Leucine-rich repeat-containing G protein-coupled receptor 4 (LGR4) plays a critical role in regulating the wingless-related integration site (Wnt) signaling pathway and is essential for organ development and carcinogenesis. LGR4, along with its ligand R-spondin (RSPO), potentiates Wnt/β-catenin signaling by recruiting its signaling suppressor, E3 ligase Zinc and Ring Finger 3 (ZNRF3), and inducing its membrane clearance. Cell surface-expressed LGR4/5, members of the class A G-protein coupled receptors (GPCR) family, have an extracellular domain (ECD) comprising 17 leucine-rich repeats (LRRs), followed by a seven-transmembrane domain (TMD), and an intracellular domain (ICD). ZNRF3/RNF43, LGR4, and RSPO form a ternary complex on the cell surface, which relieves ZNRF3/RNF43-mediated suppression of Wnt/β-catenin signaling and thereby potentiates pathway activation.

We purified LMNG/CHS detergent-solubilized ternary complexes of human LGR4, RSPO2, and ZNRF3 (residues 56-267, ECD-TMD) from Expi293F cells cotransfected with LGR4, RSPO2, and ZNRF3. Cryo-EM analysis of this sample revealed two distinct LGR4–RSPO2–ZNRF3 complexes with stoichiometric ratios of 1:1:2 and 2:2:2, corresponding to a heterotetramer and a heterohexamer, respectively. We obtained cryo-EM maps of LGR4-RSPO2-ZNRF31:1:2 heterotetramer and LGR4-RSPO2-ZNRF32:2:2 heterohexamer to resolutions of 3.2 Å and 3.5 Å, respectively. In the LGR4-RSPO2-ZNRF32:2:2 complex, another copy of the LGR4*-RSPO2* complex was bound to the other protomers of the ZNRF3 dimer, ZNRF3* (the asterisk indicates the second protomer in the dimer), forming another set of 1:1:1 complexes, thus completing the C2-symmetrical 2:2:2 complex. In the LGR4-RSPO2-ZNRF32:2:2 complex, the TM helices of ZNRF3 protomers were visible in the cryo-EM density. The two TM helices of ZNRF3 were loosely sandwiched between the two TMDs of LGR4, especially between TM1 and TM7 of one LGR4 promoter and TM6 of the other LGR4* promoter. The two TM helices of ZNRF3 made contact with each other at a distance of 5–7 Å on the extracellular side of the membrane. In addition to the ECD dimerization of ZNRF3, these intermolecular contacts in the membrane restrict the spatial positioning of the TM helices of ZNRF3 and bring the intracellular region of ZNRF3 into proximity, which may facilitate the auto-ubiquitination of ZNRF320,28,29. In the 2:2:2 heterohexamer configuration, ZNRF3 ECD and TMD are largely enclosed by LGR4 and RSPO2, resulting in steric hindrance that prevents ZNRF3 from binding to the FZDs, thereby suppressing its ubiquitination activity. Moreover, no apparent contact was observed between the two LGR4 protomers within the 2:2:2 heterohexamer.

>[2x]MPGPLGLLCFLALGLLGSAGPSGAAPPLCAAPCSCDGDRRVDCSGKGLTAVPEGLSAFTQALDISMNNITQLPEDAFKNFPFLEELQLAGNDLSFIHPKALSGLKELKVLTLQNNQLKTVPSEAIRGLSALQSLRLDANHITSVPEDSFEGLVQLRHLWLDDNSLTEVPVHPLSNLPTLQALTLALNKISSIPDFAFTNLSSLVVLHLHNNKIRSLSQHCFDGLDNLETLDLNYNNLGEFPQAIKALPSLKELGFHSNSISVIPDGAFDGNPLLRTIHLYDNPLSFVGNSAFHNLSDLHSLVIRGASMVQQFPNLTGTVHLESLTLTGTKISSIPNNLCQEQKMLRTLDLSYNNIRDLPSFNGCHALEEISLQRNQIYQIKEGTFQGLISLRILDLSRNLIHEIHSRAFATLGPITNLDVSFNELTSFPTEGLNGLNQLKLVGNFKLKEALAAKDFVNLRSLSVPYAYQCCAFWGCDSYANLNTEDNSLQDHSVAQEKGTADAANVTSTLENEEHSQIIIHCTPSTGAFKPCEYLLGSWMIRLTVWFIFLVALFFNLLVILTTFASCTSLPSSKLFIGLISVSNLFMGIYTGILTFLDAVSWGRFAEFGIWWETGSGCKVAGFLAVFSSESAIFLLMLATVERSLSAKDIMKNGKSNHLKQFRVAALLAFLGATVAGCFPLFHRGEYSASPLCLPFPTGETPSLGFTVTLVLLNSLAFLLMAVIYTKLYCNLEKEDLSENSQSSMIKHVAWLIFTNCIFFCPVAFFSFAPLITAISISPEIMKSVTLIFFPLPACLNPVLYVFFNPKFKEDWKLLKRRVTKKENLYFQGDYKDDDDKHHHHHHHH;>[2x]MQFRLFSFALIILNCMDYSHCQGNRWRRSKRASYVSNPICKGCLSCSKDNGCSRCQQKLFFFLRREGMRQYGECLHSCPSGYYGHRAPDMNRCARCRIENCDSCFSKDFCTKCKVGFYLHRGRCFDECPDGFAPLEETMECVEENLYFQGHHHHHHHHHH;>METGLRWLLLVAVLKGVQCKETAFVEVVLFESSPSGDYTTYTTGLTGRFSRAGATLSAEGEIVQMHPLGLCNNNDEEDLYEYGWVGVVKLEQPELDPKPCLTVLGKAKRAVQRGATAVIFDVSENPEAIDQLNQGSEDPLKRPVVYVKGADAIKLMNIVNKQKVARARIQHRPPRQPTEYFDMGIFLAFFVVVSLVCLILLVKIKLKQRRSQNSMNRLAVQALEKMETRKF[2x]>EVSQDLFNQFNLFAQYSAAAYCGKNNDAPAGTNITCTGNACPEVEKADATFLYSFEDSGVGDVTGFLALDNTNKLIVLSFRGSRSCE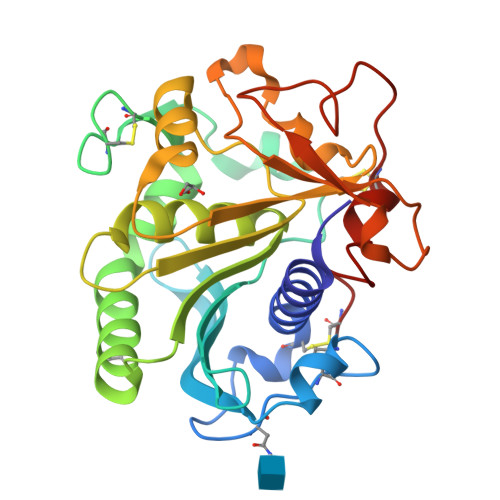NWIGNLNFDLKEINDICSGCRGHDGFTSSWRSVADTLRQKVEDAVREHPDYRVVFTGHSLGGALATVAGADLRGNGYDIDVFSYGAPRVGNRAFAEFLTVQTGGTLYRITHTNDIVPRLPPREFGYSHSSPEYWIKSGTLVPVTRNDIVKIEGIDATGGNNQPNIPDCPAHLWYFGLIGTCL[2x]> APSLLHKYMGIFFSTMSSEELLGSLDSFDAREDDIFLVSYPKSGTHWLAEVIERIPDAGI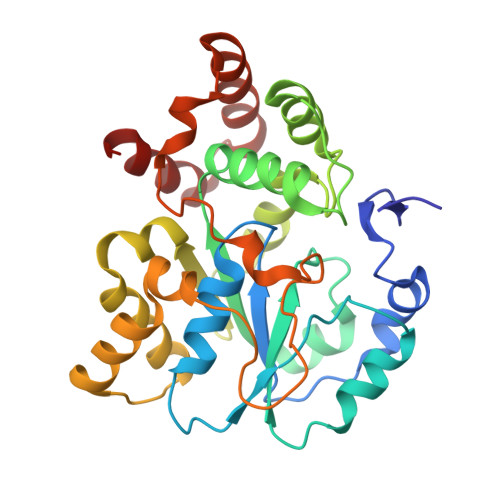TLTSPIELGDISKFEELKRIPKRRAIPTHLNYEMLPVTVKQKQCKIIYIVRNPKDTAVSMFHYYRDNPNLPSTETWAAFLELFLKGDVVYGSWFDHVLSWEEHKNDKNVLFIFYEEMKKDFVKSLKKITAFLGIDVNDSEMAKIARSTSFSEMKSNAAKENCDPNHVICALTSDRNLVFRKGVVGDWINYFTPKQNRGFDELFTEKMRNSDVGRCLKEYAHSA>HHHHHHFNLPPGNYKKPKLLYCSNGGHFLRILPDGTIDGTRDRSDQHIQLQLSAESV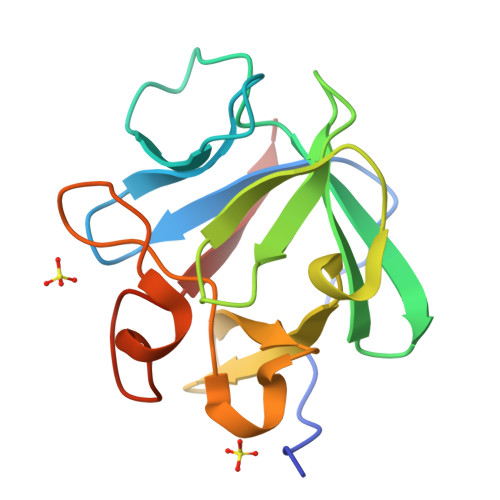GEVYIKSTETGQYLAMDTDGLLYGSQTPNEECLFLERLEENHYNTYISKKHAEKNWFVGLKKNGSCKRGPRTHYGQKAILFLPLPVSSD[2x]>[2x]MVTSLIVRLVAWSVRRPVWVVVLSLLIAAFSGVYVARHFKINTDISKLVDAEPQWAALSQAVDRAFPQRNGTILAVVEAPAPEFATAAAHALTESLQKQAAAGRIGPVAEPGGGPFFEHNGLLFLSPQQVADTTSQLASARPLVNELAKNPSLTGLATTLSTTLGQPLLTGQVKLPSMAKLLSRSAATVDDVLAGKPAAFSWRALVDNDAARQPARAFVTVQPVVNYGALKAGAQTSDVIRETARALDLEKRYGAVVRLTGEQPLADDEFSSVEDGAALNGVVTLLVVFVILWLALRSKRMIASVLVTLFVGLVVTAALGLAMVGSLNMISVAFMVLFVGLGVDFSIQYGVKYREERFRGEAIDAALIGAAHSMGMPLALATTAVAASFFSFIPTA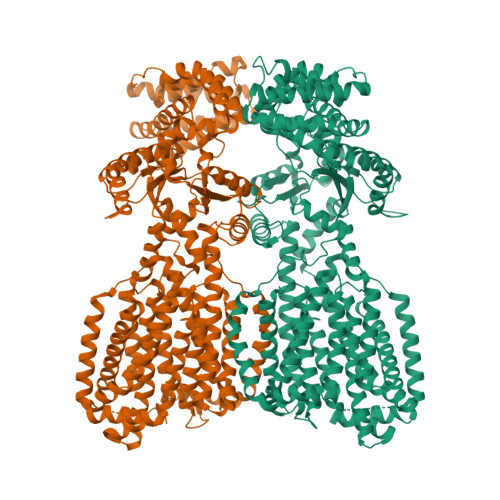YRGVSELGLIAGVGMFVALLTTLTLLPALLRLFAPPGESKTPGFPWLAPVDDYLDRHRKPILIGTLAVVIGALPLLAFLHFDFNPLHLKDPHSESMSTLLALKDSPEAAVNDVTLLAPSLADADAAAKRLDALPEVGRTTTLSTFIPADQPEKRAAIATAASTLLPALTQPPAPPATDAQRVAALKRASDLLGYAAEDHPGPGAAAAQHLSQSLAKLAAADSATRDRAERAFADTLRIALNQLAALLQPQEITRDTLPPPLVRDWVAPDGKALVQISPKVPKGVDPNDDTMLRHFATAVKAAEPGAIGGPISILHSANTIISAFLHAALWSIISITILLWITLRRFGDVLRTLVPLLVSGIVTLEMCVVLGMSLNFANIIALPLMLGVGVAFKVYFVMAWRAGQTGLLHSSLTHAVLFSAATTATAFGSLWLSHHPGTSSMGKLLALALTCTLIGAVVFQPVLMGKPRVKRAKNQSQGINEHHHHHH> GHMLRLSAPGQLDDDLCLLGDVQVPVFLLRLGEASWALVEGGISRDAELVWADLCRWVADPSQVHYWLITHKHYDHCGLLPYLCPRLPNVQV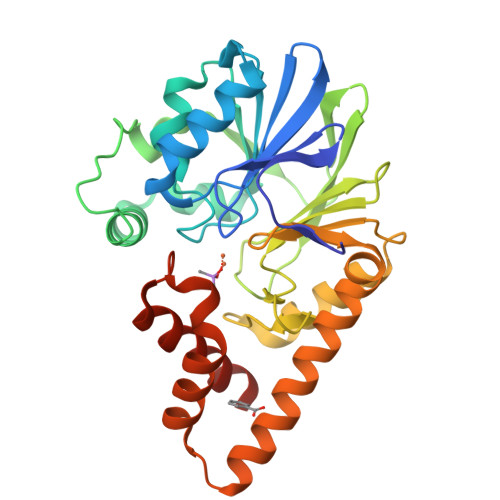LASERTCQAWKSESAVRVVERLNRQLLRAEQRLPEACAWDALPVRAVADGEWLELGPRHRLQVIEAHGHSDDHVVFYDVRRRRLFCGDALGEFDEARGVWRPLVFDDMEAYLESLERLQRLPTLLQLIPGHGGLLRGRLAADGAESAYTECLRLCRRLLWRQSMGESLDELSEELHRAWGGQSVDFLPGELHLGSMRRMLEILSRQALPLD> MKRTPLFEKHVELGAKMVDFAG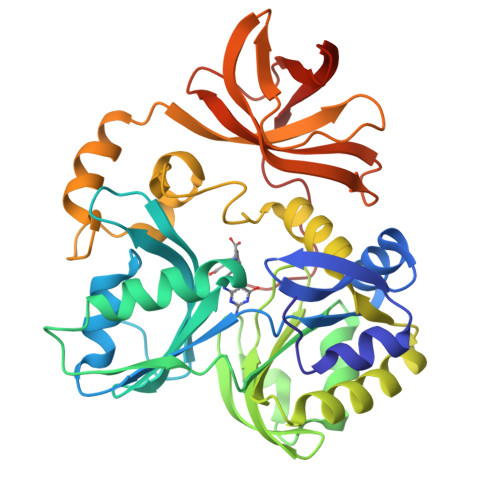WEMPLYYTSIFEEVMAVRKSVGMFDVSHMGEFLVKGPEAVSFIDFLITNDFSSLPDGKAIYSVMCNENGGIIDDLVVYKVSPDEALMVVNAANIEKDFNWIKSHSKNFDVEVSNISDTTALIAFQGPKAQETLQELVEDGLEEIAYYSFRKSIVAGVETLVSRTGYTGEDGFELMLEAKNAPKVWDALMNLLRKIDGRPAGLGARDVCRLEATYLLYGQDMDENTNPFEVGLSWVVKLNKDFVGKEALLKAKEKVERKLVALELSGKRIARKGYEVLKNGERVGEITSGNFSPTLGKSIALALVSKSVKIGDQLGVVFPGGKLVEALVVKKPFYRGSVRREV> MMKIKPVKVESIENPKRFLNSRLLTKIEVEEAIEKALKQLYINIDYFGEEYPTPATFNNIYKVMDNTEWTNGFWTGCLWLAYEYNQDKKLKNIA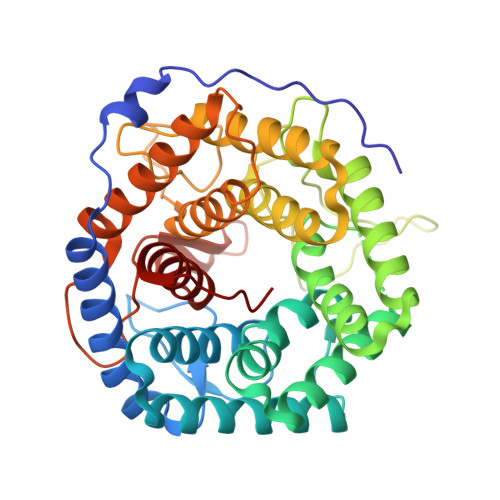HKNVLSFLNRINNRIALDHHDLGFLYTPSCTAEYRINGDVKALEATIKAADKLMERYQEKGGFIQAWGELGYKEHYRLIIDCLLNIQLLFFAYEQTGDEKYRQVAVNHFYASANNVVRDDSSAFHTFYFDPETGEPLKGVTRQGYSDESSWARGQAWGIYGIPLSYRKMKDYQQIILFKGMTNYFLNRLPEDKVSYWDLIFTDGSGQPRDTSATATAVCGIHEMLKYLPEVDPDKETYKYAMHTMLRSLIEQYSNNELIAGRPLLLHGVYSWHSGKGVDEGNIWGDYYYLEALIRFYKDWELYW>[2x]GGSMKIKQALANVYEETADWEEEITFAELIEAGLVG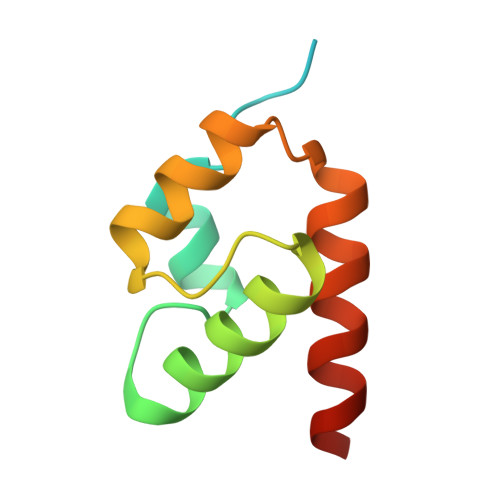GEMARRRRQRLGEELKIGYANGRQFHKRLKVFRISRDAFYAALAQVMREEAGDA>AHCIGITDRDFIEGVHGGTWVSATLEQDKCVTVMAPDKPSLDISLETVAIDRPAEVRKVCYNAVLTHVKINDKCPSTGEAHLAEENEGDNACKRTYSDRGWGNGCGLFGKGSIVACAKFTCAKSMSLFEVDQTKIQYVIRAQLHVGAKQENWNTDIKTLKFDALSGSQEVEFIGYGKATLECQVQTAVDFGNSYIAEMETESWIVDRQWAQDLTLPWQSGSGGVWREMHHLVEFEPPHAATIRVLALGNQEGSL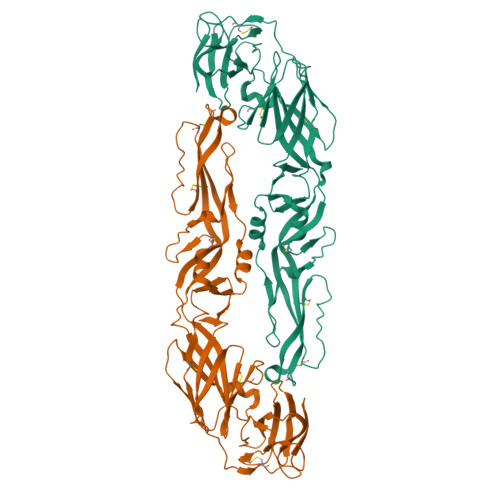KTALTGAMRVTKDTNDNNLYKLHGGHVSCRVKLSALTLKGTSYKICTDKMFFVKNPTDTGHGTVVMQVKVSKGAPCRIPVIVADDLTAAINKGILVTVNPIASTNDDEVLIEVNPPFGDSYIIVGRGDSRLTYQWHKEGSS[2x]> MFENITAAPADPILGLADLFRADERPGKINLGIGVYKDETGKTPVLTSVKKAEQYLLENETTKNYLGIDGIPEFGRCTQELLFGKGSALINDKRARTAQTPGGTGALRVAADFLAKNTSVKRVWVSNPSWPNHKSVFNSAGLEVREYAYYDAENHTLDFDALINSLNEAQAGDVVLFHGCCHAPTGIDPTLEQWQTLAQLSVEKGWLPLFDFAYQGFARGLEEDAEGLRAFAAMHKELIVASSYSKNFGLYNERVGACTLVAADSETVDRAFSQMKAAIRANYSNPPAHGASVVATILSNDALRAIWEQELTDMRQRIQRMRQLFVNTLQEKGANRDFSFIIKQNGMFSFSGLTKEQVLRLREEFGVYAVASGLVNVAGMTPD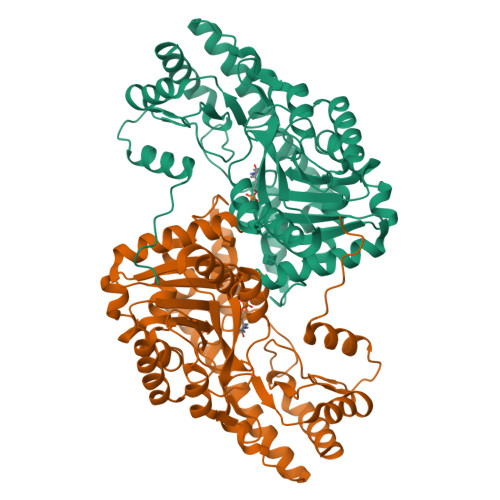NMAPLCEAIVAVL> MHHHHHHADLERRTFGSYKIEEITIKNDQQQKTTNQQQISNNEQRISTKKIPILDDGIFDLINYLLNGTHFDKTHYCGFDYSHLPTLERDFNTASNYVSENYSIIVEEIDLNKYERSESISLKSPDFTVVLEYFKKHVEGQTEQEENKTESTSSELPAKIVRELPLLPIMCRESEDSISEDILEGEGAVIQVLKMFMKGFLVHLGENPNSYDRQLTIEKYRPLLISIIGYEFTVGTRATHTKINHIYYQLATFDNYPFDLLRFQ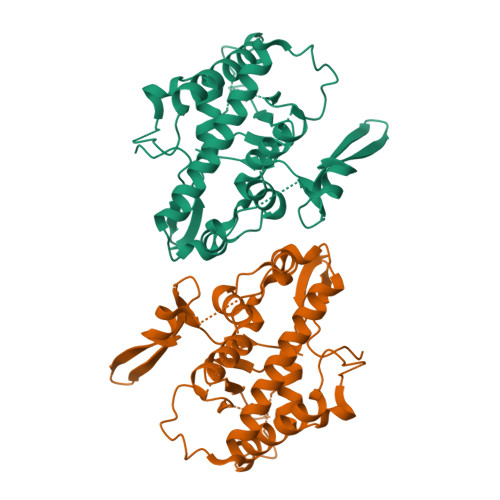LQSLIDTPNVIKERIEKDGLFKVITTTNARGQYQSVLLRGINGSESYLNLKRYRK>[4x]MGSSHHHHHHSQDLENLYFQGSQINQVRPKLPLLKIL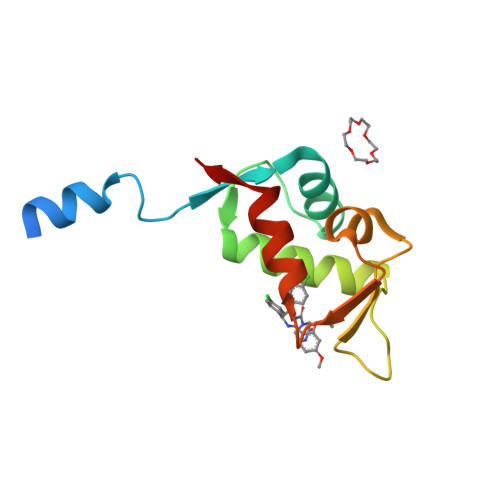HAAGAQGEMFTVKEVMHYLGQYIMVKQLYDQQEQHMVYCGGDLLGELLGRQSFSVKDPSPLYDMLRKNLVTLAT In this work, we exhaustively probe the ability of all 36 immobile HJ sequences to form DNA crystals in two different designed systems. Three separate self-assembling DNA crystal systems are described in this report: the “4 × 5” and “4 × 6” designs (collectively referred to as the 4 × N systems), and a third construct with a “scrambled” sequence variant of the 4 × 6 lattices. Self-assembly was mediated by three constituent oligonucleotides: (S1) containing four sequence repeats of either 5 or 6 bases; (S2) composed of 21 bases containing complementary regions to both (S1); and (S3) which forms the second junction crossover. The HJ serves as the fundamental component at the core of each unit, and the ultimate assembly of the full lattice is facilitated by the complementary 2-base sticky ends that tail each duplex.

Because the 4 × 6 system yielded R3 symmetry in 5 of 17 junctions, we considered whether the downstream sequences adjacent to the junction could play a role in crystallization efficiency, junction angle, and symmetry preference, or if the HJ alone was the singular determinant. To investigate this possibility, we designed “scrambled” sequences with targeted base substitutions, while maintaining GC content, along each “stem”. Contrary to the buffer preference observed with the native P32 crystals, the scrambled systems exhibited an exclusive preference towards low salt buffers, much like the native R3 crystals. Remarkably, only J1 and J2 retained the P32 symmetry, with all others yielding an R3 lattice. There appeared to be only a marginal difference in the average cell lengths in the R3 scramble crystals (a = b = 113.04 c = 51.10) relative to the native 4 × 6 sequences: the a, b axis trended ~2 Å shorter and c ~1.3 Å longer, whereas in the J1 and J2 cases, the crystals were in good agreement with the original 4 × 6 motif. The average angles of the R3 and P32 crystals were 61.00° (σ = 1.21) and 58.05° (σ = 1.39), respectively. Further, we observed modest improvements in resolution, reaching as high as 2.7 Å in J36. Notably, all junctions preventing crystallization compared to its original counterpart remained fatal and all relative cavity dimensions and volumes remained unperturbed. Another major observation is the importance of stem region sequences outside the HJ, given that this sequence can control crystal symmetry and lattice architecture, and improve resolution in non-obvious ways.

> GAACGACACTGA;> CGTGGACTC;> TCAACG;> TCGAGTCCGTGTCGT> SGRPMTLQSAMGDMYQSIFVATPPLLQMEQEQPFPELIRTWAGLLGQIGVESVRTEEVNFGQLAKCFNDYLNTVAEHCEQQNIWQHKREENHNFFTAFKPDASKAALHGHAYIAHYKESVILRHLSIVDPKTLGMLRFAPYEAPSTDYCRHFPDSPWAKMQRLA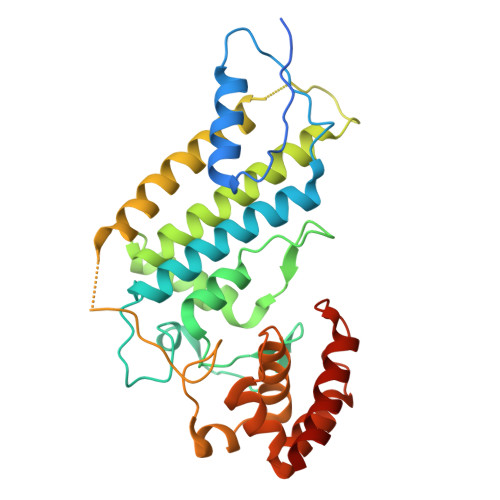TAGQNIILQLRLIQNGQMLEDDFMKEKLPVLQKALDDFMQYKTEVDALLAHDSEVTPVSTHDSSFFYDIDEQTLNAMSGDQLATICFEELNAPHPSRLIMRILKSDSLWQEVDDSLNGDAFMGRQDDICEKRNKICQWRQLVQMTT> CGVGFIANLRGKPDHTLVEQALKALGCMEHRGGCSADNDSGDGAGVMTAIPRELLAQWFNTRNLPMPDGDRLGVGMVFLPQEPSAREVARAYVEEVVRLEKLTVLGWREVPVNSDVLG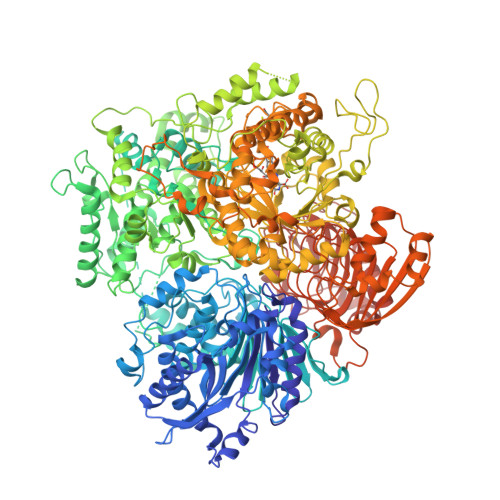IQAKNNQPHIEQILVTCPEGCAGDELDRRLYIARSIIGKKLAEDFYVCSFSCRTIVYKGMVRSIILGEFYLDLKNPGYTSNFAVYHRRFSTNTMPKWPLAQPMRLLGHNGEINTLLGNINWMAAREKELEVSGWTKAELEALTPIVNQANSDSYNLDSALELLVRTGRSPLEAAMILVPEAYKNQPALKDYPEISDFHDYYSGLQEPWDGPALLVFSDGKIVGAGLDRNGLRPARYCITKDDYIVLGSEAGVVDLPEVDIVEKGRLAPGQMIAVDLAEQKILKNYQIKQQAAQKYPYGEWIKIQRQTVASDSFAEKTLFNDAQTVLQQQAAFGYTAEDVEMVVVPMASQGKEPTFCMGDDTPLAVLSHKPRLLYDYFKQRFAQVTNPPIDPLRENLVMSLAMFLGKRGNLLEPKAESARTIKLRSPLVNEVELQAIKTGQLQVAEVSTLYDLDGVNSLEDALTNLVKTAIATVQAGAEILVLTDRPNGAILTENQSFIPPLLAVGAVHHHLIRAGLRLKASLIVDTAQCWSTHHFACLVGYGASAICPYLALESVRQWWLDEKTQKLMENGRLDRIDLPTALKNYRQSVEAGLFKILSKMGISLLASYHGAQIFEAIGLGAELVEYAFAGTTSRVGGLTIADVAGEVMVFHGMAFPEMAKKLENFGFVNYRPGGEYHMNSPEMSKSLHKAVAAYKVGGNGNNGEAYDHYELYRQYLKDRPVTALRDLLDFNADQPAISLEEVESVESIVKRFCTGGMSLGALSREAHETLAIAMNRLGAKSNSGEGGEDVVRYLTLDDVDSEGNSPTLPHLHGLQNGDTANSAIKQIASGRFGVTPEYLMSGKQLEIKMAQGAKPGEGGQLPGKKVSEYIAMLRRSKPGVTLISPPPHHDIYSIEDLAQLIYDLHQINPEAQVSVKLVAEIGIGTIAAGVAKANADIIQISGHDGGTGASPLSSIKHAGSPWELGVTEVHRVLMENQLRDRVLLRADGGLKTGWDVVMAALMGAEEYGFGSIAMIAEGCIMARVCHTNNCPVGVATQQERLRQRFKGVPGQVVNFFYFIAEEVRSLLAHLGYRSLDDIIGRTDLLKVRSDVQLSKTQNLTLDCLLNLPDTKQNRQWLNHEPVHSNGPVLDDDILADPDIQEAINHQTTATKTYRLVNTDRTVGTRLSGAIAKKYGNNGFEGNITLNFQGAAGQSFGAFNLDGMTLHLQGEANDYVGKGMNGGEIVIVPHPQASFAPEDNVIIGNTCLYGATGGNLYANGRAGERFAVRNSVGKAVIEGAGDHCCEYMTGGVIVVLGPVGRNVGAGMTGGLAYFLDEVGDLPEKINPEIITLQRITASKGEEQLKSLITAHVEHTGSPKGKAILANWSDYLGKFWQAVPPSEKDSPEANNDVSLTGEKTLTSV>APAKKDASEVKRSKVEIIKEKSNFLRYPLNEELVSEAPNINESAVQLIKFHGSYQQTDRDVRGQKNYSFMLRTKNPCGKVPNQLYLAMDTLADEFGIGTLRLTTRQTFQLHGVLKKNLKTVLSTVIKNMGSTLGACGDLNRNVLAPAAPYVKKDILFAQQTAENIAALLTPQSGAYYDLWVDGEKIMSAEEPPEVTKARNDNSHGTNFPDSPEPIYGTQYLPRKFKVAVTAAGDNSVDILTNDIGVVVVSDDAGEPIGFNIYVGGGMGRTHRVETTFPRLADPLGYVPKEDILYAIKAIVVTQRENGRRDDRKYSRMKYMIDRWGIDRFRAEVEKYYGKKFESFRPLPEWQFNSYLGWQEQGDGKLFYGVHVDNGRVGGQAKKTLREIIEKYNLDVSITPNQNLILCGIDQ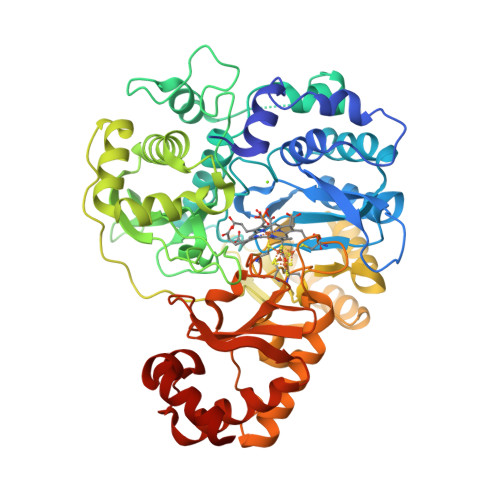AWREPITTALAQAGLLEPKDVDPLNLTAMACPALPLCPLAQTEAERGILPILKRIRAVFNKVGIKDSESVVVRITGCPNGCARPYMAELGFVGDGPKSYQIWLGGTPNQSTLAESFMDKVKLDDIEKVLEPLFTYWNGTRQEGESFGSFTNRTGFDKLKEVVNKWAESPSAA[2x]>MKHHHHHHPMVMLNVGATAPDFTLRDQNQQLVTLRGYRGAKNVLLVFFPLAFTGICQGELDQLRDHLPEFENDDSAALAIS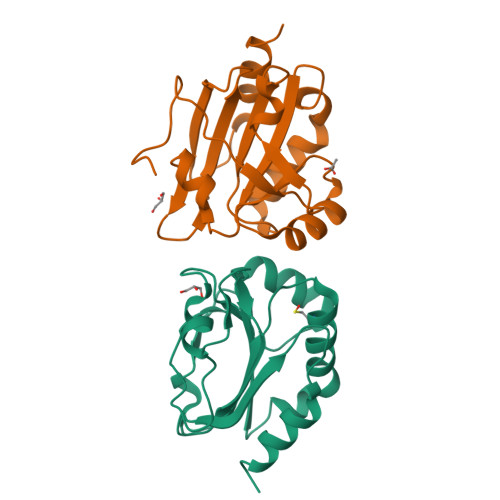VGPPPTHKIWATQSGFTFPLLSDFWPHGAVSQAYGVFNEQAGIANRGTFVVDRSGIIRFAEMKQPGEVRDQRLWTDALAALTA[4x]>MKLKTNIRHLHGIIRVPGDKSISHRSIIFGSLAEGETKVYDILRGEDVLSTMQVFRDLGVEIEDKDGVITVQGVGMAGLKAPQNALNMGNSGTSIRLISGVLAGADFEVEMFGDDSLSKRPMDRVTLPLKKMGVSISGQTERDLPPLRLKGTKNLRPIHYELPIASAQVKSALMFAALQAKGESVIIEKEYTRNHTEDMLQQFGGHLSVDGKKITVQGPQKLTGQKVVVPGDISSAAFWLVAGLIAPNSRLVLQNVGINETRTGIIDV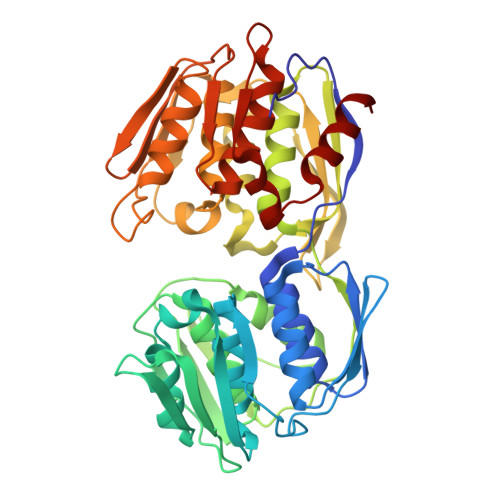IRAMGGKLEITEIDPVAKSATLIVESSDLKGTEICGALIPRLIDELPIIALLATQAQGVTVIKDAEELKVKETDRIQVVADALNSMGADITPTADGMIIKGKSALHGARVNTFGDHRIGMMTAIAALLVADGEVELDRAEAINTSYPSFFDDLESLIHG[4x]(5R)-5-(4-methoxyphenyl)-5-(3-pyrimidin-5-ylphenyl)-3,4-dihydropyrrol-2-amine | C21 H20 N4 O | 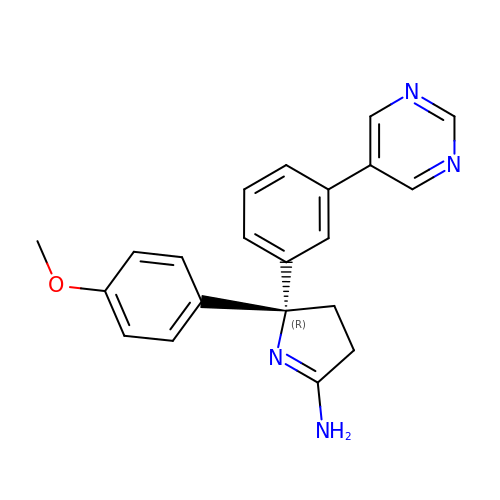MLDNPVIFXVSEGX-OAQYLSRUSA-N> G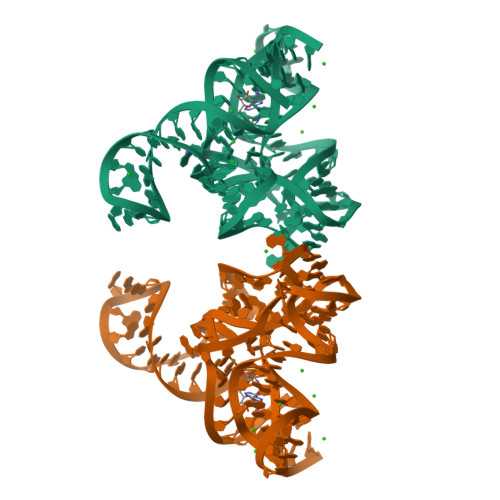GCUUAUCAAGAGAGGGAGAGCGACUGGCGCGAAGAACCCCGGCAACCAGAAAUGGUGCCAAUUCCUGCAGCGGAAACGUUGAAAGAUGAGCCG> GAMSDATPFRPPSEAEEALIKETRLPLTGWQQEVDQGLTYGLEAAASIKDRSIPTFSRGELPHYAGINTFMKAPYLEDVREVGKYDVAIVGVPH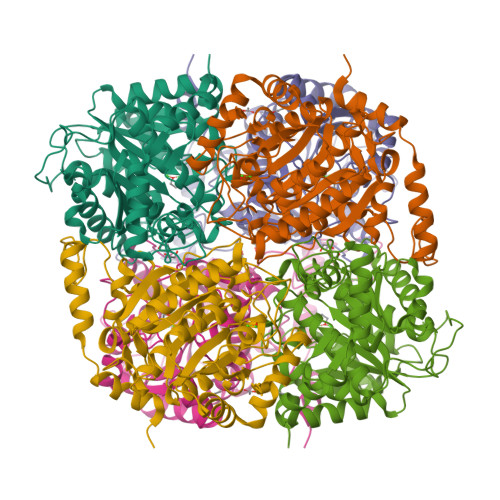DSGTTYRPGTRFGPQGIRRISALYTPYNFEMGVDLREQISLCDVGDIFTIPANNEKSFDQISKGIAHIFSSGAFPIILGGDHSIGFPTVRGICRHLGDKKVGIIHFDRHVDTQETDLDERMHTCPWFHATNMANAPAKNLVQLGIGGWQVPRQGVKVCRERATNILTVTDITEMSLDAAADFAIARATDGTDCVWISFDIDCIDAGFVPGTGWPEPGGLLPREALYLLKRIIRETNVCGMEVVEVSPPYDISDMTSLMATRVICDTMAHLVVSGQLPRTEKPAYIHAEANMAVDEPWQ>[5x]GDRVADVIESSIGDSVSRALTHALPAPTGQNTQVSSHRLDTGKVPALQAAEIGASSNASDES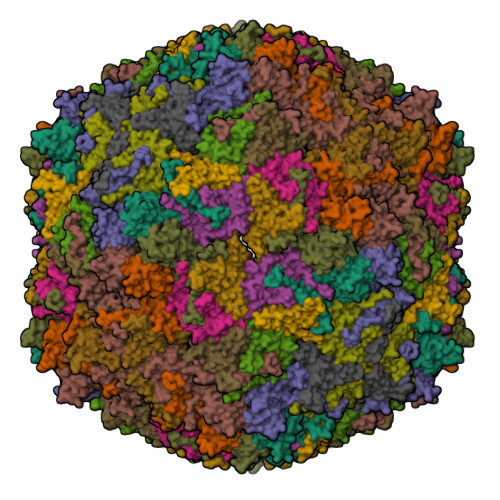MIETRCVLNSHSTAETTLDSFFSRAGLVGEIDLPLEGTERKRARLTPNGYANWDIDITGYAQMRRKVELFTYMRFDAEFTFVACTPTGEVVPQLLQYMFVPPGAPKPDSRESLAWQTATNPSVFVKLSDPPAQVSVPFMSPASAYQWFYDGYPTFGEHKQEKDLEYGACPNNMMGTFSVRTVGTSKSKYPLVVRIYMRMKHVRAWIPRPMRNQNYLFKANPNYAGNSIKPTGASRTAITTL;>[5x]GFPTELKPGTNQFLTTDDGVSAPILPNFHPTPCIHIPGEVRNLLELCQVETILEVNNVPTNATSLMERLRFPVSAQAGKGELCAVFRADPGRSGPWQSTLLGQLCGYYTQWSGSLEVTFMFTGSFMATGKMLIAYTPPGGPLPKDRATAMLGTHVIWDFGLQSSVTLVIPWISNTHYRAHARDGVFDYYTTGLVSIWYQTNYVVPIGAPNTAYIIALAAAQKNFTMQLCKDASDILQTGTIQ;>MGSQVSTQRSGSHENSNSATEGSTINYTTINYYKDSYAATAGKQSLKQDPDKFANPVKDIFTEMAAPLKSPSAEACGYSDRVAQLTIGNSTITTQEAANIIVGYGEWPSYCSDSDATAVDKPTRPDVSVNRFYTLDTKLWEKSSKGWYWKFPDVLTETGVFGQNAQFHYLYRSGFCIHVQCNASKFHQGALLVAVLPEYVIGTVAGGTGTEDSHPPYKQTQPGADGFELQHPYVLDAGIPISQLTVCPHQWINLRTNNCATIIVPYINALPFDSALNHCNFGLLVVPISPLDYDQGATPVIPITITLAPMCSEFAGLRQAVTQ[5x]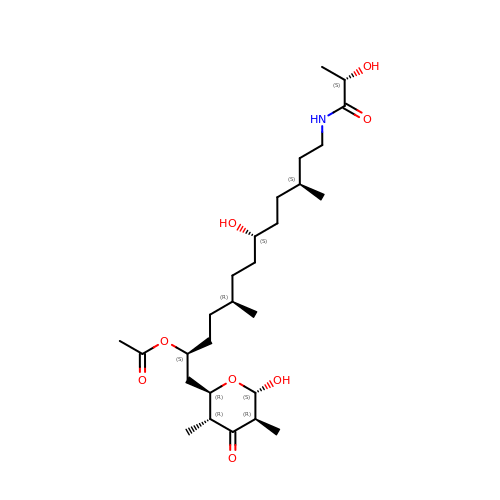[(2~{S},5~{R},8~{S},11~{S})-1-[(2~{R},3~{R},5~{R},6~{S})-3,5-dimethyl-6-oxidanyl-4-oxidanylidene-oxan-2-yl]-5,11-dimethyl-8-oxidanyl-13-[[(2~{S})-2-oxidanylpropanoyl]amino]tridecan-2-yl] ethanoate | C27 H49 N O8 | OEJUFLVQZDMQAY-BVGDNXMFSA-N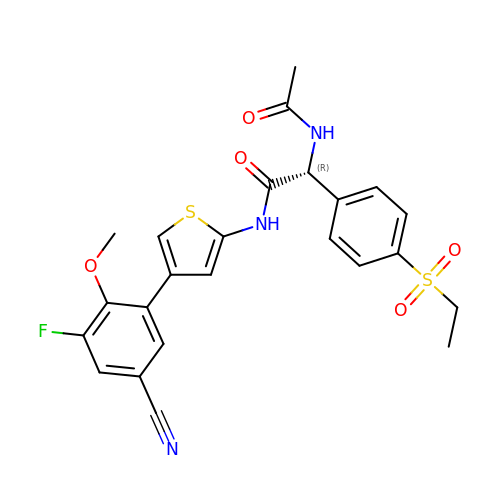(2~{R})-2-acetamido-~{N}-[4-(5-cyano-3-fluoranyl-2-methoxy-phenyl)thiophen-2-yl]-2-(4-ethylsulfonylphenyl)ethanamide | C24 H22 F N3 O5 S2 | YOJMBDUWFJVSKK-JOCHJYFZSA-N> MSQHKATYQQHIEELQARTREALQREGLDGLVIHSGQGKRLFLDDNHYPFKVNPQFKAWVPVIDNPNCWLVVNGVDKPTLIFYRPEDFWHKVPPEPNDFWTDSFDIKLLQQADAVEKFLPYDKSRFAYVGEYIEVAKALGFDNVNPDRVLHYLHYQRAYKTDYELDCMREANKLAVAGHKAAEQAFREGKSEFDINLAYAAASRQGDNDVPYTS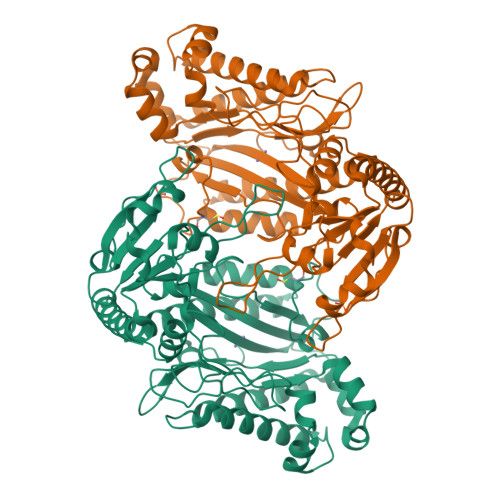IVALNEHASILHYMQCDTVAPKESRSFLIDAGANYHGYAADITRTYAQEGVHNSAMFRDLIQAVDKVTLTLVDSLKPGVAYTDIHLLAHDGIAQILHDTGMVNLTPPEIVEMGITRTFFPHGIGHFLGLQVHDVGGLVNDDRGTPKPAPDDHPFLRCTRMVEARQVFTIEPGLYFIDSLLRDLKATPASKYINWDTIDAYKPFGGIRIEDNIIVHRDKNENMTRDLDLNLEHHHHHH>GSHPVSSLTMLNDTLHNIRTTNQALKK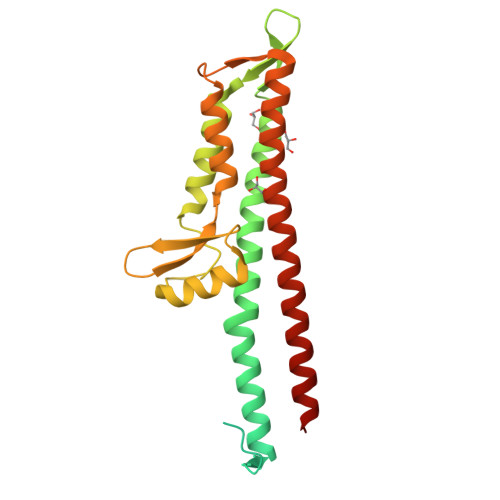ELSQKTLTKTSLEEIALHSSQISMDVNKSAQLLDILSRNEYPINKDARELLHSAPKEAELDGDQMISHRELWAKIANSINDINEQYLKVYEHAVSSYTQMYQDFSAVLSSLAGWISPGGNDGNSVKLQVNSLKKALEELKEKYKDKPLYPANNTVSQEQANKWLTELGGTIGKVSQKNGGYVVSINMTPIDNMLKSLDNLGGNGEVVLDNAKYQAWNAGFSAEDETMKNNLQTLVQKYSNANSIFDNLVKVLSSTISSS[2x]>[3x]SDLIPAPPLSKVPLQQNFQDNQFHGKWYVVGF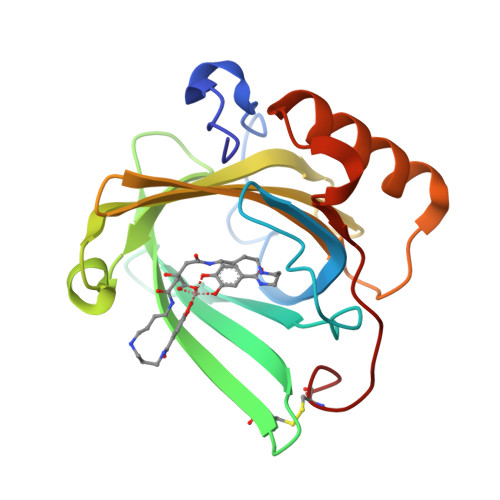AENIQQREDKDPPKMIATIYELKEDKSYNVTNVASNWEKCTYRIKTFVPGSQPGEFTLGEIKSRPGMTSYLVRVVSTNYNQHAMVFFKTVVQNREKFWITLYGRTKELTSELKENFIRFSKSLGLPENHIVFPVPIDQCIDG>PSVYDAAAQLTADVKKDLRDSWKVIGSDKKGNGVAAMTTLFADNQETIGYFKRLGDVSQGMANDKLRGHSITLMYALQNFIDQLDNPDDLVCVVEKFAVNHITRKISAAEFGKINGP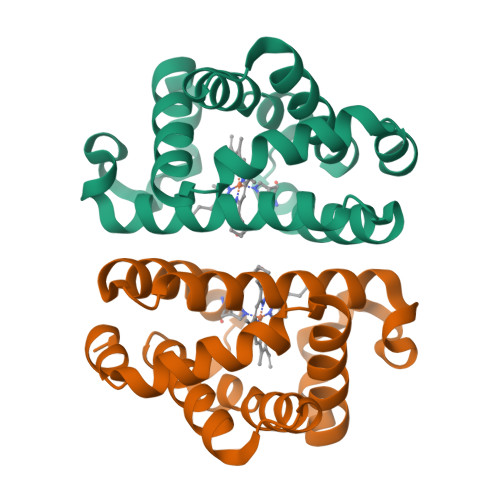IKKVLASKNFGDKYANAWAKLVAVVQAAL[2x]>[2x]GGGG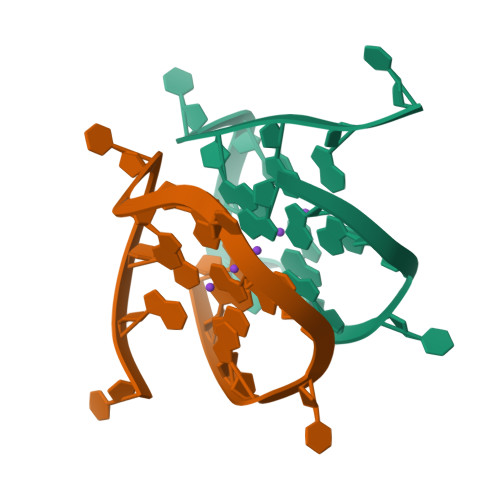TGGGTGGTGGGT> KDMQLAR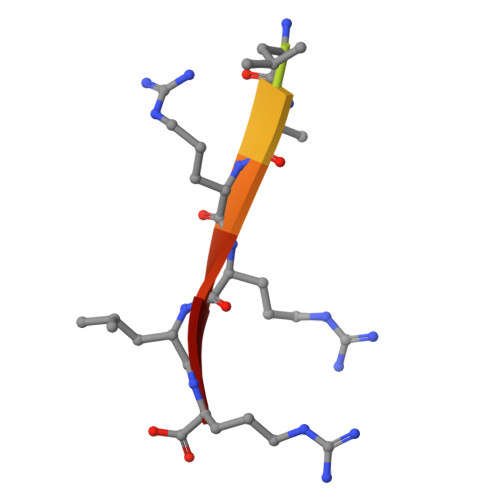RLR Aureothin 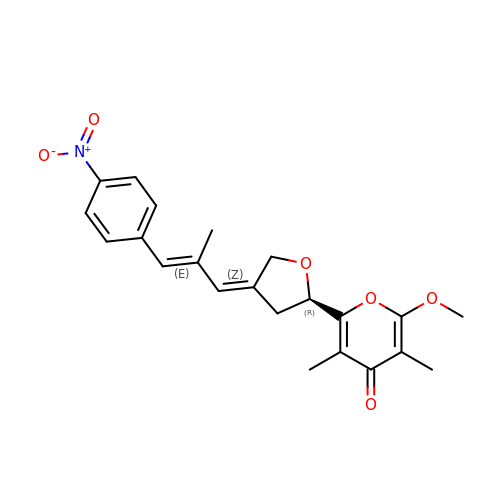| C22 H23 N O6 | GQKXCBCSVYJUMI-WACKOAQBSA-N>MENKQKLKRPIQRIVRLSEEENNLIKRKIEESFFPNFQNFALHLLIQGEIRHVDYSELNRLTTEIHKIGININQMARLANQFHEISSEDIKDLTDKVQSLNALVQSELNKLIKRK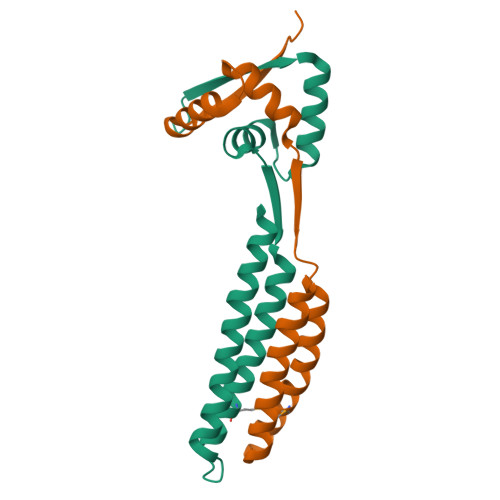DQS[4x]1-[3-(naphthalen-1-yloxy)propyl]-5,6-dihydro-4H-pyrrolo[3,2,1-ij]quinoline-2-carboxylic 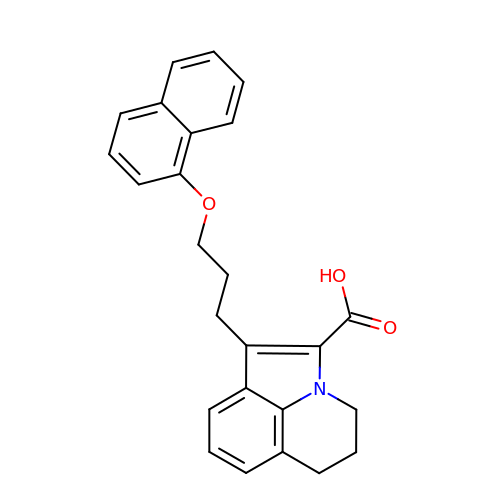acid | C25 H23 N O3 | XOMAOOTVWOCYAD-UHFFFAOYSA-N> MGHHHHHHENLYFQGMKKEKVEQILAEFQLQEEDLKKVMRRMQKEMDRGLRLETHEEASVKMLPTYVRSTPEGSEVGDFLSLDLGGTNFRVMLVKVGEGEEGQWSVKTKHQMYSIPEDAMTGTAEMLFDYISECISDFLDKHQMKHKKLPLGFTFSFPVRHEDIDKGILLNWTKGFKASGAEGNNVVGLLRDAIKRRGDFEMDVVAMVNDTVATMISCYYEDHQCEVGMIVGTGCNACYMEEMQNVELVEGDEGRMCVNTEWGAFGDSGELDEFLLEYDRLVDESSANPGQQLYEKLIGGKYMGELVRLVLLRLVDENLLFHGEASEQLRTRGAFETRFVSQVKSDTGDRKQIYNILSTLGLRPSTTDCDIVRRACESVSTRAAHMCSAGLAGVINRMRESRSEDVMRITVGVDGSV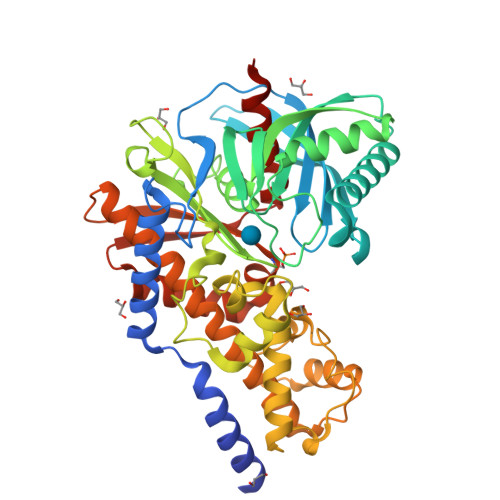YKLHPSFKERFHASVRRLTPSCEITFIESEEGSGRGAALVSAVACKKACMLGQ> MTGGMKPPARKPRILNSDGSSNITRLGLEKRGWLDDHYHDLLTVSWPVFITLITGLYLVTNALFALAYLACGDVIENARPGSFTDAFFFSVQTMATIGYGKLIPIGPLANTLVTLEALCGMLG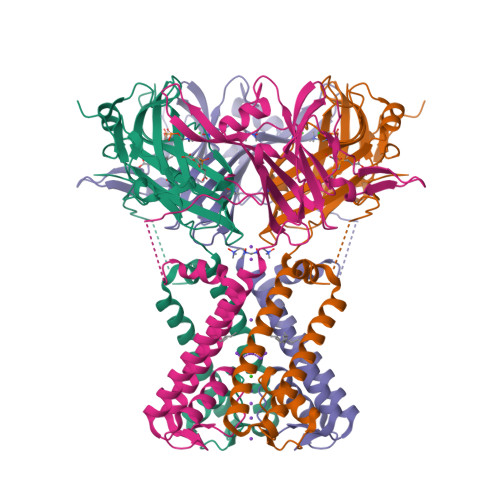LAVAASLIYARFTRPTAGVLFSSRMVISDFEGKPTLMMRLANLRIEQIIEADVHLVLVRSEISQEGMVFRRFHDLTLTRSRSPIFSLSWTVMHPIDHHSPIYGETDETLRNSHSEFLVLFTGHHEAFAQNVHARHAYSCDEIIWGGHFVDVFTTLPDGRRALDLGKFHEIAQHHHHHH> MLDAFSRVVTNADSKAAYVGGADLQALKKFISEGNKRLDAVNSIVSNASCIV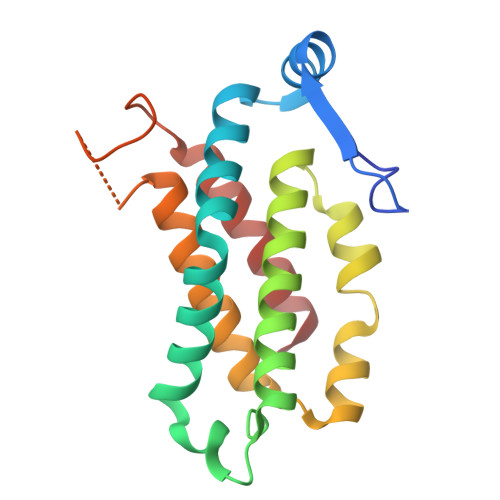SDAVSGMICENPSLISPSGNCYTNRRMAACLRDAEIILRYVSYALLSGDSSVLEDRCLNGLKETYSSLGVPANGNARAVSIMKACSVAFVNNTASQKKLSTPQGDCSGLASEVAGYFDKVTSAIS> MAPTSSSTKKTQLQLEHLLLDLQMILNMLNNYDNPKLTRLLTFKFYMPKKATSLKHLQCLEEELKPLEEALNAAGDDPKTIRDVVSNINVFVLELKGSETTFMCEYADETATIIEFLNRWITFC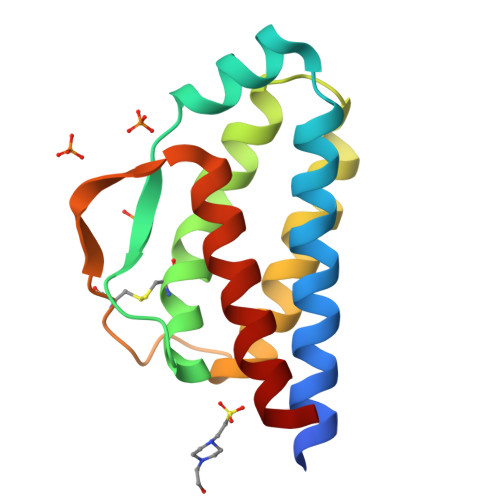QSIISTLT> GELVRTDSPNFLCSVLPTHWRCNKTLPIAFKVVAKGDVPDGTLVTVMAGNDENYSAELRNATAAMKNQVARFNDLRFVGRSGRGKSFTLTITVFTNPPQVATYHRAIKITADGPREPRRHRQKLDDQTKPG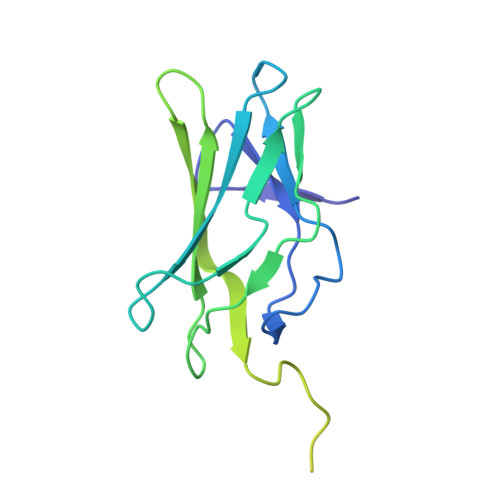SLSFSERLSELEQLRRTAMRVSPHHPAPTPNPRASLNHSTAFNPQPQSQMQDARQIQPSPPWSYDQSYQYLGS> MMRSSSFCRRQIRPYYNLPSKSEHGRKMTGFLTPYRHWMWKQNELWRNVHEAQFEHLRRVYKRQWLESFRVNADEYIYKYNITKAAQLAQWECEMKEQEKKRIEARQMMDGRQALKKKHLDLLREFHERQFFFWYERASERLQNMNLINYVP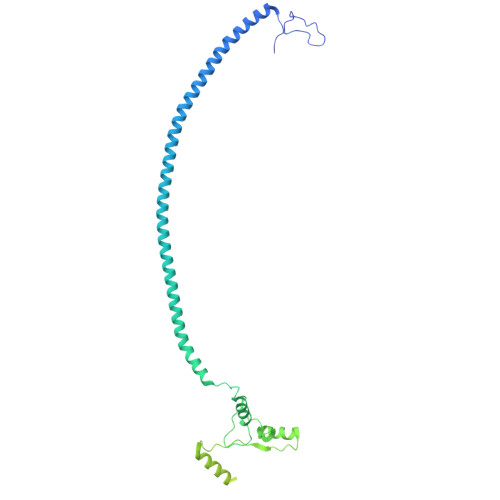HAQLREHIDKELDKYVAGKNEPYPLNFVGQMPFLEDGDGNIVEVPESLLSNHMAEHPDSTAKPHEPHTSSSISEAAAFEERMLRAMVSAKEEDLKEWLGDDSRALSETIDDISREEEEREADIRVARSMEETDAEREVSRRAYIERXKTGSRSIFRPPTVSEGAGGTPSAPAGDANTPMRRRKKGKLDRVHALQAHQDELLAKLSSQGLKEXVDASSVPERGKIVQSRGRIRDKAVIPTHEVLMQKPELAAGSTPGARIQTKDMVDKMYHRGKYKKSGSGDKSDGEDL> GRQVKTETYTNTVTNVP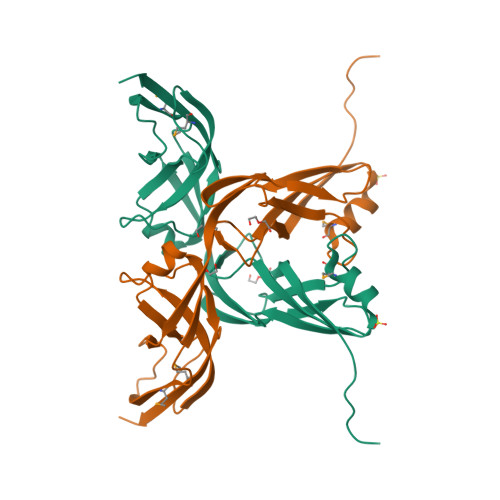IDIRYNSDKYFISGFASEVSVVLTGANRLSLASEMQESTRKFKVTADLTDAGVGTIEVPLSIEDLPNGLTAVATPQKITVKIGKKAQKDKVKIVPEIDPSQIDSRVQIENVMVSDKEVSITSDQETLDRIDKIIAVLPTSERITGNYSGSVPLQAIDRNGVVLPAVITPFDTIMKVTTKPVAPSSSTSNSSTSSSSETSSSTKATSSKTN> AISIKTPEDIEKMRVAGRLAAEVLEMIEPYVKPGVSTGELDRICNDYIVNEQHAVSACLGYHGYPKSVCISINEVVCHGIPDDAKLLKDGDIVNIDVTVIKDGFHGDTSKMFIVGKPTIMGERLCRITQESLYLALRMVKPGINLREIGAAIQKFVEAEGFSVVREYCGHGIGQ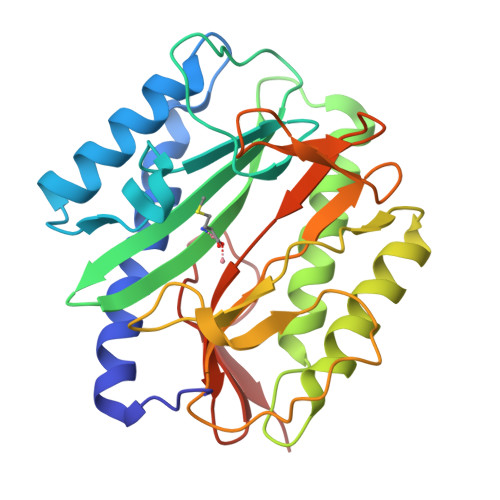GFHEEPQVLHYDSRETNVVLKPGMTFTIEPMVNAGKKEIRTMKDGWTVKTKDRSLSAQYEHTIVVTDNGCEILTLRKDDTIPAIISHDE>GKAVIAIHGGAGAISRAQMSLQQELRYIEALSAIVETGQKMLEAGESALDVVTEAVRLLEECPLFNAGIGAVFTRDETHELDACVMDGNTLKAGAVAGVSHLRNPVLAARLVMEQSPHVMMIGEGAENFAFARGMERVSPEIFSTSLR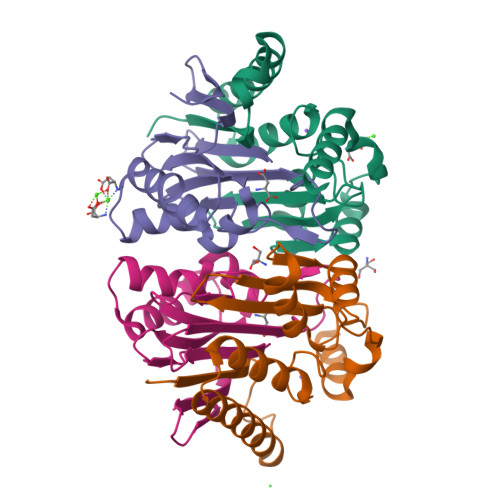YEQLLAARKEGA[2x];>[2x]TVGAVALDLDGNLAAATSTGGMTNKLPGRVGDSPLVGAGCYANNASVAVSCTGTGEVFIRALAAYDIAALMDYGGLSLAEACERVVMEKLPALGGSGGLIAIDHEGNVALPFNTEGMYRAWGYAGDTPTTGIYREKG> AAATTCTCTACTGTGG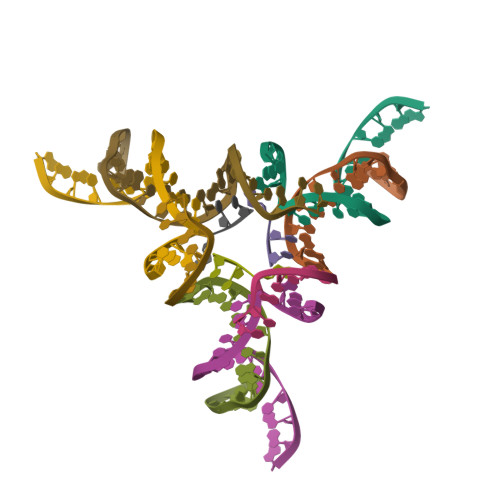AT;> TCATCCT;> GGACAGTAGAGAAT;> ACC>MKDIAIRGYCDRPSVATGETIRFYVSANETRGTFDAELVRLIHGDSNPAGPGYKEEAIKSDLEGQYPARFQRTQFGSYVEVADPDAGLQPDGAFSVHLFLWSTTPSRGRQGIASRWNDERQSGWNLAIEDGRVVFTIGDGSGATSSVVSDRPLFQQIWYSITGVYDPEKKQLRLYQKSVVNRTNSRFGLVVPLDSDCAVSADATVKAADSETSLLIAGLGEAAAQDGRTWCIAHYNGKVDAPKIYGCALGQDDAEKLSRGEIVRPISRLAHWDFSAGIGLNGIPTDHVVDASGYGHHGRCMNQPSRGSTGWNWDGHEENFIHCPEQYGALWFHEDCLDDCRWEKDFEFTVPEGLKSDFYAVKIRYEDTEDYIPFFVLPPRGTATAPILVIASTLSYLAYANEQIMHKADIGQAVAGHTPVLNENDVELHKNLSYYGLSTYDGHIDGRGVQYTSWRRPIMNLRPKHRQGFGSIWELPADLHLIDWLNHNGFEYDVATEHDLNDQGAELLRRYKVVLTGSHPEYQTWANADAWEDYLADGGRGMYLAANGMYWIVEVHPEKPWVMEVRKELGVTAWEAPPGEYHYSTNGRRGGRFRGR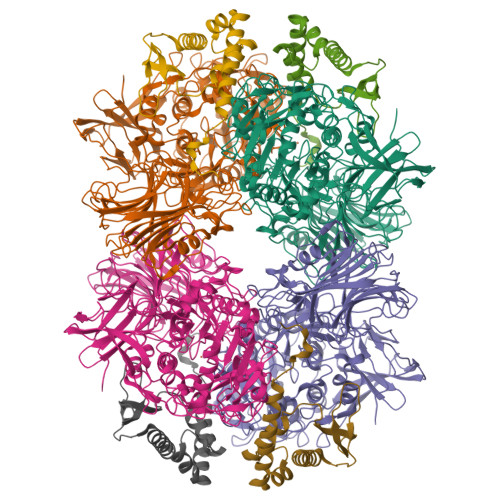ARATQKIWGTGMSSFGFDHSGYFVQMPDSQDERVAWIMEGIDPEERIGDGGLVGGGAGGYELDRYDLALGTPPNTLLLASSVEHSVVYTVIPDDKAFPHPGMNGGEHPFVRADITYFSTANGGGMFATSSISWLGSLSWNDYDNNVSKMTKNVLNQFIKDEPAPRVKLAAALEHHHHHH[4x];>[4x]MTEASESCVRDPSNYRDRSADWYAFYDERRRKEIIDIIDEHPEIVEEHAANPFGYRKHPSPYLQRVHNYFRMQPTFGRYYIYSEREWDAYRIATIREFGELPELGDERFKTEEEAMHAVFLRRIEDVRAELA>MGQGNDTSEVMLLDTGWEFSQSGTEKWMPATVPGTVHQDLISHELLPNPFYGMNEKKIQWVENEDWEYRTSFIVSEEQLNRDGIQLIFEGLDTYADVYLNGSLLLKADNMFVGYTLPVKSVLRKGENHLYIYFHSPIRQTLPQYASNGFNYPADNDHHEKHLSVFSRKAPYSYGWDWGIRMVTSGVWRPVTLRFYDIATISDYYVRQLSLTDENARLSNELIVNQIVPQKIPAEVRVNVSLNGTTVTEVKQQVTLQPGINHITLPAEVTNPVRWMPNGWGTPTLYDFSAQIACGDRIVAEQSHRIGLRTIRVVNEKDKDGESFYFEVNGIPMFAKGANYIPQDALLPNVTTERYQTLFRDMKEANMNMVRIWGGGTYENNLFYDLADENGILVWQDFMFACTPYPSDPTFLKRVEAEAVYNIRRLRNHASLAMWCGNNEILEALKYWGFEKKFTPEVYQGLMHGYDKLFRELLPSTVKEFDSDRFYVHSSPYLANWGRPESWGTGDSHNWGVWYGKKPFESLDTDLPRFMSEFGFQSFPEMKTIAAFAAPEDYQIESEVMNAHQKSSIGNSLIRTYMERDYIIPESFEDFVYVGLVLQGQGMRHGLEAHRRNRPYCMGTLYWQLNDSWPVVSWSSIDYYGNWKALHYQAKRAFAPVLINPIQQNDSLSVYLISDRLDTMEQMTLEMKVVDFDGKTLGKKIQVHSLEVPANTSKCVYRAKLDGWLTPEDCRRSFLKLILKDKSGHQVAESVHFFRKTKDLQLPPTSVSYQMKQTDGKCELTLFSSMLAKDIFIETPLQGARYSDNFFDLLPGERKKVIITSPRIKKGEELPVNIKHIRETYKLEHHHHHH[2x]

Exo-β-mannosidases, hydrolysing non-reducing terminal β-d-mannopyranosidic linkages, are widely distributed carbohydrate-degrading enzymes. All of these exo-β-mannosidases process their substrate using a stereochemically retaining double displacement mechanism that is characterised by the formation of a covalent glycosyl enzyme intermediate (GEI). We show that these probes covalently label exo-β-mannosidases from GH families 2, 5, and 164. Structural studies of the resulting complexes support a canonical mechanism-based mode of action in which the active site nucleophile attacks the pseudoanomeric centre to form a stable ester linkage, mimicking the glycosyl enzyme intermediate.

No significant inhibition of BtMan2A could be detected following incubation with 1 or 2, but the enzyme was 85% inhibited by 3, again indicating performance enhancement attributable to the N-octylazido linker. The electron density for several aromatic residues lining the entrance to the active site pocket, notably W470, W533, and Y537 were extremely diffuse, hindering modelling and suggesting a high degree of mobility in the complex. The alkyl linker extends into a channel lined with these diffuse aromatic residues, possibly giving rise to similar, albeit more dynamic, hydrophobic interactions to those observed in the CmMan5A active site. Comparisons of the labelled enzyme structure to the previously determined structures of complexes with 2,4-dinitrophenyl 2-deoxy-2-fluoro-β-d-mannoside (2FMan, non-covalent/pre-catalytic) and noeuromycin, show that the ligand has migrated significantly away from the expected position of the GEI (ESI Fig. 3†). Reorientation of the catalytic nucleophile breaks the hydrogen bond with O2, allowing relaxation of the ring conformation. This makes space for a water molecule to interact with R393. Due to the interaction of these aromatic rings with the alkyl linker, we hypothesized that hydrophobic interactions related to the presence of the octyl linker drive this active site rearrangement. We thus conclude that there exists a more fundamental instability in the GEI structure of BtMan2A, possibly explaining earlier failures to trap it.N-(phenylcarbonyl)-beta-alanine | C10 H11 N O3 | 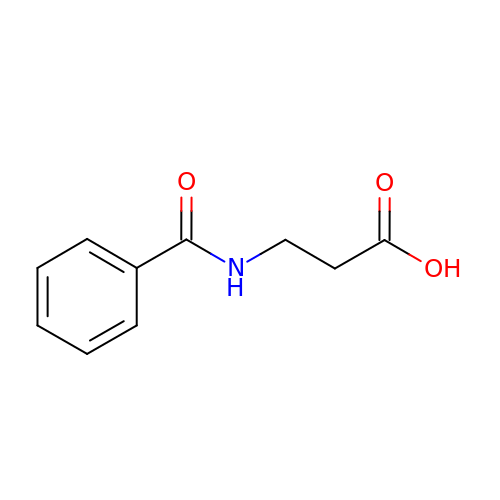CWXYHOHYCJXYFQ-UHFFFAOYSA-N> SNAERALLQLVVEDDAKALVFVLGQDARRYFEEELPASPFEFPSPQAVA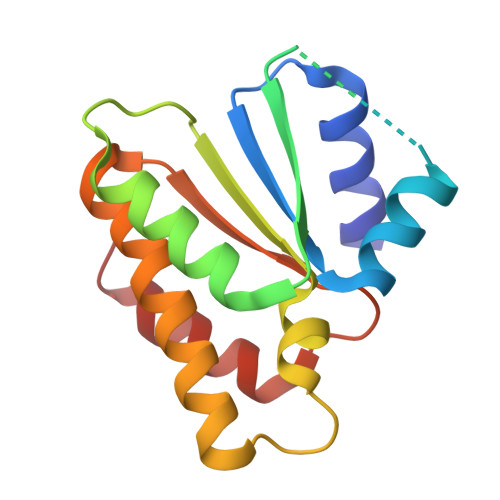NSRQNVGVMFLDKLQYLYMYLTKLEVDEAPEYRTLVVYGLEQLLGAGGELDADQVRLASLIYNTAFRVRVRHGAAVRFVAHGAPHAQLQQLEAHWRLFT>MSTHIGEPQDSYTEEIPQDERRFTRLDKGVASPGSVTVSGNRKTVQAPASGIIKNIAVRDGDKVKAGEVLVQLSQVQAQAQVDSLRDQYYTTLATEGRLLAERDGLSIVTFSPILDAVKDKPRVAEIIALQTQLFASRRQALQSEIDGYKQSMDGIRFQLKGLQDSRGNKQIQLSSLREQMNSMKQLAADGYLPRNRYLEVQRQFAEVNSSIDETVGRIGQLQKQLLESQQRIDQRFADYQREVRTQLAQTQMDASEFRNKLQMADFDLGNTAITSPVDGTVVGLNIFTQGGVVGAGDHLMDVVPSQATLVVDSRLKV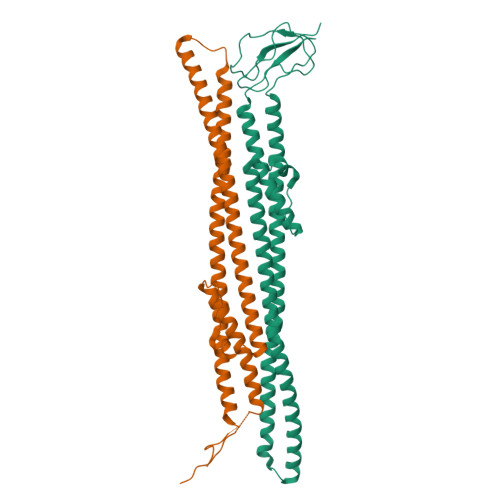DLFDKVYNGLPVDLMFTAFNQNKTPKIPGTVTLVSADRLVDKANGEPYYQMQVTVSPEGMKMLSGEDIKPGMPVEVFVKTGSRSLLSYLFKPILDRAHTSLTEELEIKRASQPELAPEDPEDVEHHHHHH[2x]>[2x]MTSLRDLIPKHKFDNSTIDQLCKLIDNEIEPIIFDLLKWLQDYNWPIAKDILPVVVLHQSIAMPHILTILQGNDIMWKYWVIKLMIPYLIYPNKQLVKSELERLSSLEIINEDIREIVNLSKDYLHFYYP

Cthe_2751_is a 15.8 kDa singleton from an anaerobic, hyperthermophile Clostridium thermocellum, with an unknown function. Therefore, based on primary sequence analysis, Cthe_2751 is a non-Pfam singleton with an unknown function. Each monomer is made up of 8 α-helices arranged in a spiral pattern around a vertical axis that runs through the centre of the protein. The structure reveals an all α-helical topology similar to those observed for nucleic acid processing proteins.

We have solved the 3-D structure of the non-Pfam singleton Cthe_2751 to 2.17 Å resolution by Se-SAD. The 2.17 Å crystal structure of Cthe_2751 in space group P212121 consists of α-helices and loops with no β-strands. Cthe_2751 crystallized as a dimer in 3 different crystal forms. Superimposition of the dimers crystallized in different space groups revealed no obvious differences in the position of the Cα atoms suggesting an identical mode of dimerization in all the 3 crystal forms. The analysis revealed that dimerization occurs via a large area that spans 904 Å2 (12.8%) of the surface area per monomer. Interestingly, the aromatic ring of Tyr88 from one monomer protrudes into a concave cavity formed by Leu52, Pro53, Leu84 and Tyr88 of another monomer, zipping the monomers together. As for the crystal form P212121, the packing arrangement of the dimers clearly deviates from those found in space groups C2221 and P4122. There is a 60.9° orientation difference between the corresponding dimer in P212121 and that in other two space groups (C2221 and P4122). As expected, the inter-dimer distance between 2 closest dimers in space groups C2221 and P4122 is relatively similar when compared to that of the distance between dimers of space groups P212121 and C2221 or P212121 and P4122, where there is almost no recognizable co-relationship.Tripartite ATP-independent periplasmic (TRAP) transporters are secondary transporters that have evolved an obligate dependence on a substrate-binding protein (SBP) to confer unidirectional transport. We investigated the significance of this interaction using the sialic acid-specific SBP, SiaP, from the Haemophilus influenzae virulence-related SiaPQM TRAP transporter. The first structure of a TRAP SBP revealed that the charge of the carboxylate group of the ligand, sialic acid, was neutralized by an arginine residue, Arg-147, in SiaP, which sequence analysis had revealed to be the most highly conserved residue, being present in 98% of TRAP SBPs of the common DctP family. Using in vitro, in vivo, and structural methods applied to SiaP, we demonstrate that the coordination of the acidic ligand moiety of sialic acid by the conserved arginine (Arg-147) is essential for the function of the transporter as a high affinity scavenging system.

To understand the structural consequences of removing the Arg-147 from SiaP, we crystallized the R147A and R147K mutants in the presence of 10–15 mm Neu5Ac. Surprisingly, given the very weak binding observed for these proteins in vitro, both structures contain Neu5Ac bound in the substrate binding pocket, and the proteins are clearly in the closed ligand-bound conformation as opposed to the expected open ligand-free conformation that has been observed for SiaP previously. With the relatively conservative substitution of arginine to an also charged lysine, the key guanidinium group of Arg-147 is partially substituted by the Nζ atom of Lys-147, which occupies an equivalent position (0.3 Å shift) to one of the NH2 groups of Arg-147 and provides one of the interactions with the ligand. The other contact is now mediated by a water molecule that provides the missing H-bond to the carboxylate of Neu5Ac. One of these water molecules (water 1) is present in both the R147K and R147A structures, although the other water (water 3) is unique to this structure. The Arg-147 mutations were introduced into the F170W background, and we were able to detect saturable Neu5Ac binding to the F170W/ R147K mutant alone with very low affinity (KD of 38.7 ± 8.3 mm). Rapid uptake of 5 μm [14C]Neu5Ac into these cells was observed for the wild-type siaP allele, whereas no detectable uptake was observed with the R147A allele but a very low level of uptake for the R147K allele was detected (inset). Interestingly, we observed differential growth phenotypes for the Arg-147 mutants, with the more conservative changes in the R147K mutant exhibiting growth more similar to the strain expressing the wild-type SiaP (doubling times of ∼120 min), than the R147A mutation, which resulted in an ∼50% decrease in the growth rate, giving a doubling time of about ∼180 min.

> ADYDLKFGMNAGTSSNEYKAAEMFAKEVKEKSQGKIEISLYPSSQLGDDRAMLKQLKDGSLDFTFAESARFQLFYPEAAVFALPYVISNYNVAQKALFDTEFGKDLIKKMDKDLGVTLLSQAYNGTRQTTSNRAINSIADMKGLKLKVPNAATNLAYAKYVGASPTPMAFSEVYLALQTNAVDGQENPLAAVQAQKFYEVQKFLAMTNHILNDQLYLVSNETYKELPEDLQKVVKDAAENAAKYHTKLFVDGEKDLVTFFEKQGVKITHPDLVPFKESMKPYYAEFVKQTGQKGESALKQIEAINPHH>[2x]GPPFTPNEIKNKEFSRVKNGLEPTEVANFLEQLSTEIERLKEDKKQLEKVI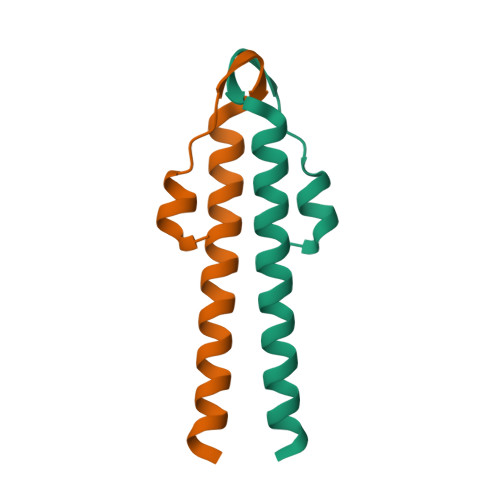EERDTNIK> GSMEYEWKPDEQGLQQILQLLKESQSPDTTIQRTVQQKLEQLNQYPDFNNYLIFVLTKLKSEDEPTRSLSGLILKNNVKAHFQNFPNGVTDFIKSECLNNIGDSSPLIRATVGILITTIASKGELQNWPDLLPKLCSLLDSEDYNTCEGAFGALQKICEDSAEILDSDVLDRPLNIMIPKFLQFFKHSSPKIRSHAVACVNQFIISRTQALMLHIDSFIENLFALAGDEEPEVRKNVCRALVMLLEVRMDRLLPHMHNIVEYMLQRTQDQDENVALEACEFWLTLAEQPICKDVLVRHLPKLIPVLVNGMKYSDIDIILLKGDVEEDETIPDSEQDIRGGSGGSGDTISDWNLRKCSAAALDVLANVYRDELLPHILPLLKELLFHHEWVVKESGILVLGAIAEGCMQGMIPYLPELIPHLIQCLSDKKALVRSITCWTLSRYAHWVVSQPPDTYLKPLMTELLKRILDSNKRVQEAACSAFATLEEEACTELVPYLAYILDTLVFAFSKYQHKNLLILYDAIGTLADSVGHHLNKPEYIQMLMPPLIQKWNMLKDEDKDLFPLLECLSSVATALQSGFLPYCEPVYQRCVNLVQKTLAQAMLNNAQPDQYEAPDKDFMIVALDLLSGLAEGLGGNIEQLVARSNILTLMYQCMQDKMPEVRQSSFALL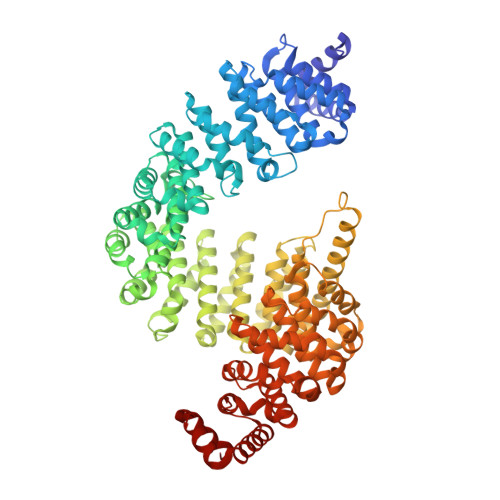GDLTKACFQHVKPCIADFMPILGTNLNPEFISVCNNATWAIGEISIQMGIEMQPYIPMVLHQLVEIINRPNTPKTLLENTAITIGRLGYVCPQEVAPMLQQFIRPWCTSLRNIRDNEEKDSAFRGICTMISVNPSGVIQDFIFFCDAVASWINPKDDLRDMFCKILHGFKNQVGDENWRRFSDQFPLPLKERLAAFYGV> MATGTRYAGKVVVVTGGGRGIGAGIVRAFVNSGARVVICDKDESGGRALEQELPGAVFILCDVTQEDDVKTLVSETIRRFGRLDCVVNNAGHHPPPQRPEETSAQGFRQLLELNLLGTYTLT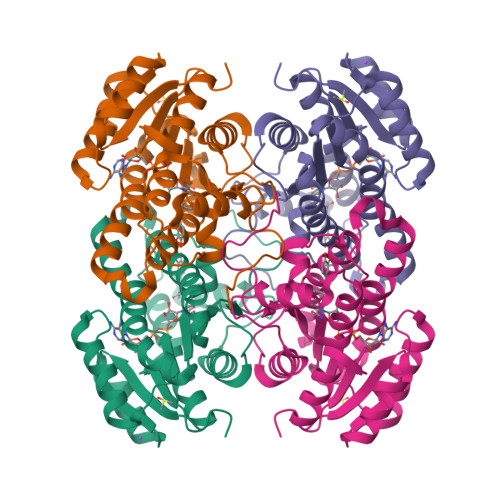KLALPYLRKSQGNVINISSLVGAIGQAQAVPYVATKGAVTAMTKALALDESPYGVRVNCISPGNIWTPLWEELAALMPDPRASIREGMLAQPLGRMGQPAEVGAAAVFLASEANFCTGIELLVTGGAELGYGAKASRSTPVDAPDIPS>[4x]GSEGQLTLLLGKLMTLLGDVSLSQLESRLAVWQAMIESQKEMGIQVSKEFQTALGEAQEATDLYEASIKKTDTAKSVYD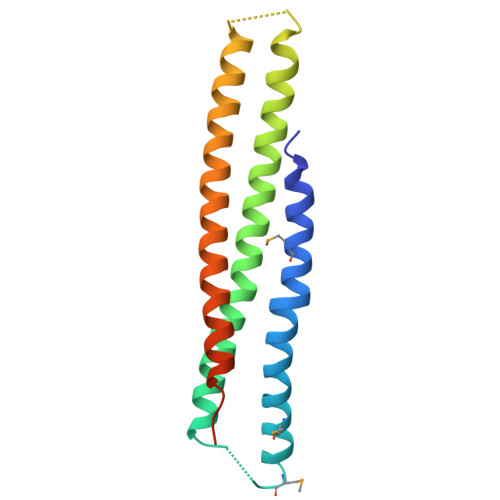AATKKLTQAQNKLQSLDPADPGYAQAEAAVEQAGKEATEAKEALDKATDATVKAGTDAKAKAEKADNILTKFQGTANAA>SMKLTIPELSLVVLIGSSGSGKSTFAKKHFKPTEVISSDFCRGLMSDDENDQTVTGAAFDVLHYIVSKRLQLGKLTVVDATN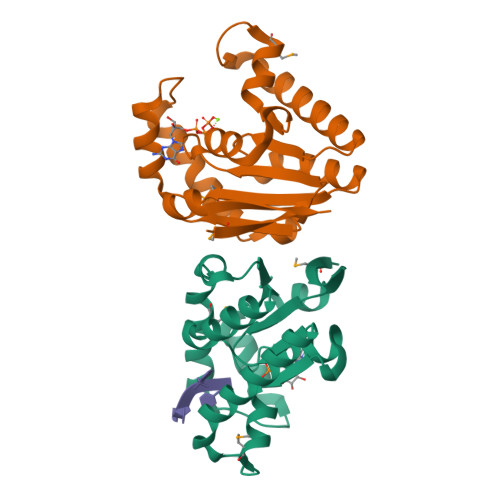VQESARKPLIEIAKDYHCFPVAVVFNLPEKVCQERNKNRTDRQVEEYVIRKHTQQMKKSIKGLQREGFRYVYILNSPEEVEEVVFERQP[2x]> TPASGALLQQMNLASQSLNYELSFISINKQGVE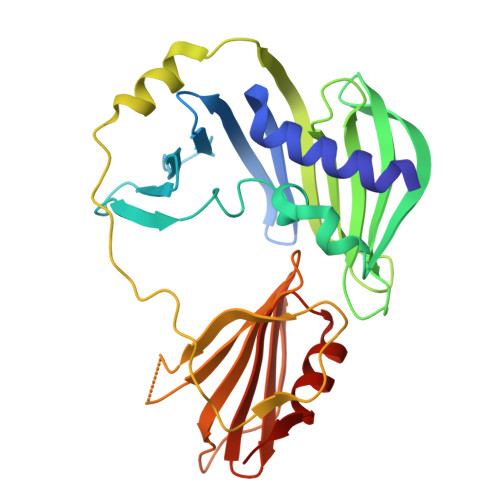SLRYRHARLDNRPLAQLLQMDGPRREVVQRGNEISYFEPGLEPFTLNGDYIVDSLPSLIYTDFKRLSPYYDFISVGRTRIADRLCEVIRVVARDGTRYSYIVWMDTESKLPMRVDLLDRDGETLEQFRVIAFNVNQDISSSMQTLAKANLPPLLSVPVGEKAKFSWTPTWLPQGFSEVSSSRRPLPTMDNMPIESRLYSDGLFSFSVNVNRATPSSTDQMLRTGRRTVSTSVRDNAEITIVGELPPQTAKRIAENIKFGAAQ> MLSAARLQFAQGSVRRLTVSARDAPTKISTLAVKVHGGSRYATKDGVAHLLNRFNFQNTNTRSALKLVRESELLGGTFKSTLDREYITLKATFLKDDLPYYVNALADVLYKTAFKPHELTESVLPAARYDYAVAEQCPVKSAEDQLYAITFRKGLGNPLLYDGVERVSLQDIKDFADKVYTKENLEVSGENVVE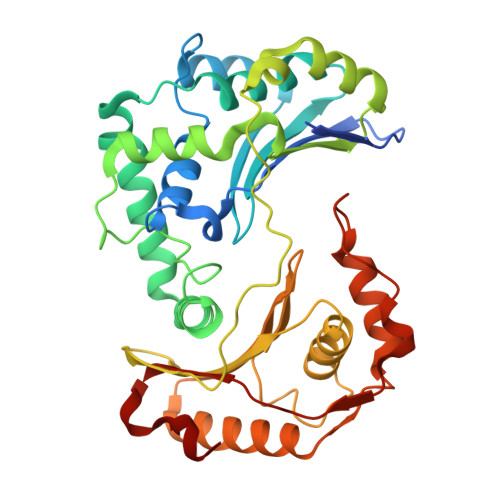ADLKRFVDESLLSTLPAGKSLVSKSEPKFFLGEENRVRFIGDSVAAIGIPVNKASLAQYEVLANYLTSALSELSGLISSAKLDKFTDGGLFTLFVRDQDSAVVSSNIKKIVADLKKGKDLSPAINYTKLKNAVQNESVSSPIELNFDAVKDFKLGKFNYVAVGDVSNLPYLDEL>[12x]MKTINSVDTKEFLNHQVANLNVFTVKIHQIHWYM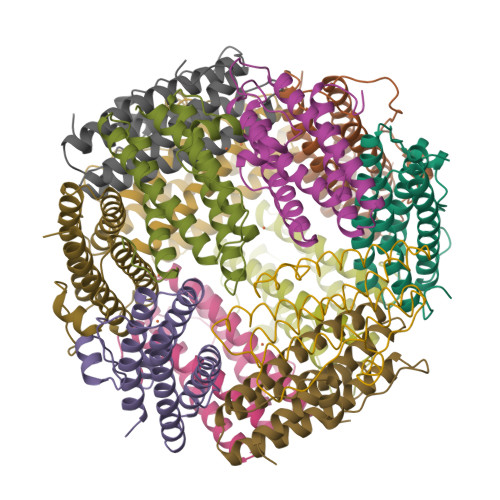RGHNFFTLHEKMDDLYSEFGEQMDEVAERLLAIGGSPFSTLKEFLENASVEEAPYTKPKTMDQLMEDLVGTLELLRDEYKQGIELTDKEGDDVTNDMLIAFKASIDKHIWMFKAFLGKAPLE> MPVDRILEAELAVEQKSDQGVEGPGGTGGSGSSPNDPVTNICQAADKQLFTLVEWAKRIPHFSSLPLDDQVILLRAGWNELLIASFSHRSIDVRDGILLATGLHVHRNSAHSAGVGAIFDRVLTELVSKMRDMRMDKTELGCLRAIILFNPDAKGLSNPSEVEVLREKVYASLETYCKQKYPEQQGRFAKLLLRLPALRSIGLKCLEHLFFFKLIGDTPIDTFLMEMLEAPHQLA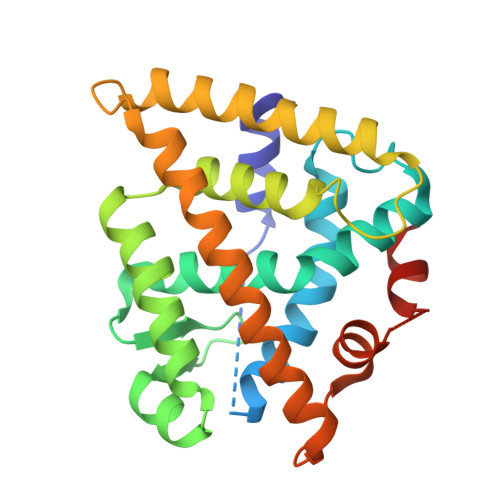GSGSGSHKILHRLLQDSSS> MRD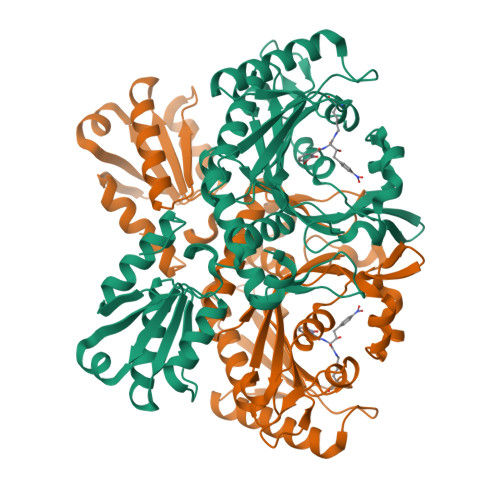HRKIGKQLDLYHMQEEAPGMVFWHNDGWTIFRELEVFVRSKLKEYQYQEVKGPFMMDRVLWEKTGHWDNYKDAMFTTSSENREYCIKPMNCPGHVQIFNQGLKSYRDLPLRMAEFGSCHRNEPSGSLHGLMRVRGFTQDDAHIFCTEEQIRDEVNGCIRLVYDMYSTFGFEKIVVKLSTRPEKRIGSDEMWDRAEADLAVALEENNIPFEYQLGEGAFKGPKIEFTLYDCLDRAWQCGTVQLDFSLPSRLSASYVGEDNERKVPVMIHRAILGSMERFIGILTEEFAGFFPTWLAPVQVVIMNITDSQSEYVNELTQKLSNAGIRVKADLRNEKIGFKIREHTLRRVPYMLVCGDKEVESGKVAVRTRRGKDLGSMDVNEVIEKLQQEIRSRSLKQLEELEHHHHHH>[3x]MRGSHHHHHHGSMASSFSMEKVKRILDAQRTEGPATVLAIGTANPPTCFYEADYPDFYFRVTNCEDKPELKEKFKRISERSAVKKRYLHVTEEILKENPNMCSYRAPSLDARHAILVEEVPKLGKEAALKAIKEWGQPLSKITHLIFSAMSGVDIPGADFRLMNLLGLEPSVNRLMIYTQGCYMGGAAMRHAKDIAENNAGARVLLVFCDLMDMYFHAPQNRVDLLYGQAVFGDGAAALIVGA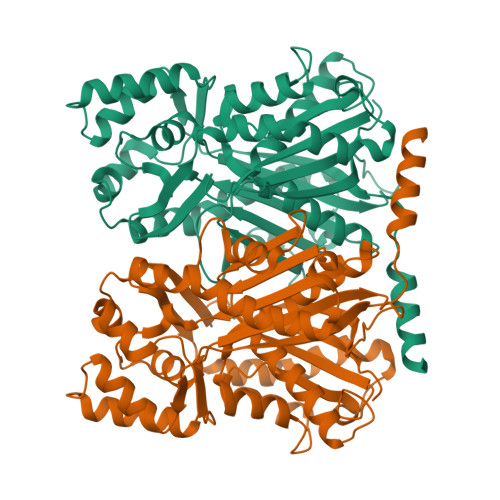DPDDDCTERPLFQVVSCAERAVPGTQDYIKAHLKEMGMELHLSTDVPRMIGKNIEKLLADAVSPFGISDWNSLFYIVHPGAVAILDQVEENLGLGEDKLRASRYVLSEYGNMGAASVFFILDEMRNKSAEEGKLTTGEGLEWGVLFSFGPGLTVETVVLLSVPLDSNH> GGSLGTLLDYAAGVIPASQIRAAGAVGAIRYVSDRRPGGAWMLGKPIQLSEARDLSGNGLKIVSCYQYGKGSTADWLGGASAGVQHARRGSELHAAAGGPTSAPIYASIDDNPSYEQYKNQIVPYLRSWESVIGHQRTGVY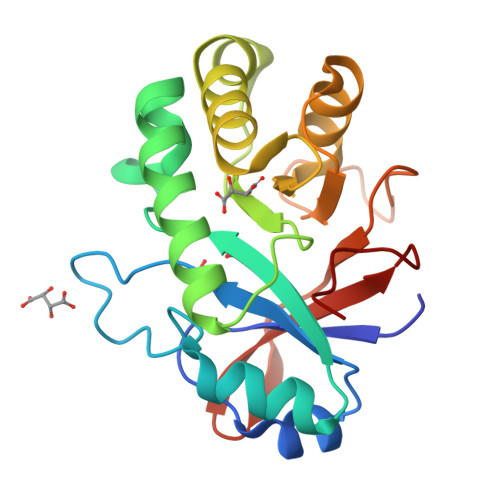ANSKTIDWAVNDGLGSYFWQHNWGSPKGYTHPAAHLHQVEIDKRKVGGVGVDVNQILKPQFGQWA>[2x]GSFKFTAQQHVYDINGVKVGGQPGEYPTVLIGSIFYRGHKIVSDGQKGIFDKDAAKALLDQEAELSAETGNPFIIDVLGESVEALTKYVEFILENTTAPFLLASISPDVRVGALKNLGKDPEIQKR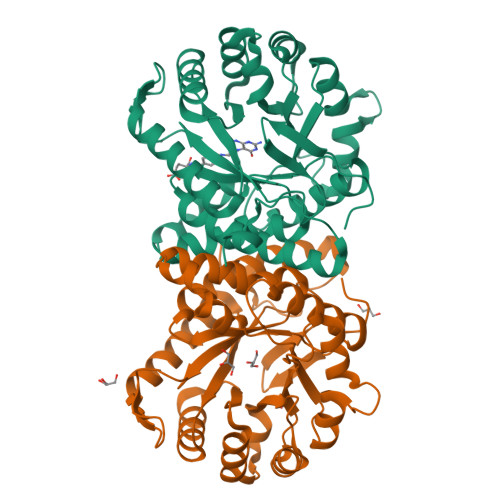LIYNSIEEHYTEEELAAIKEAGLKTAVILAFSKKALKPNARIDLLQGKDDKEGLIAAAKRAGIEQFLVDPGVLDVASNSWTTEAINVVKEQFGYPGGCAPSNAVYLWKKMRSKGTPFFEVAGAAVFTYPITQGADFILYGPMMNAPWVYRAIATTDAMIAYNNKLTGVKMGTTEHPLLKIF> MLQFYRNLGKSGLRVSCL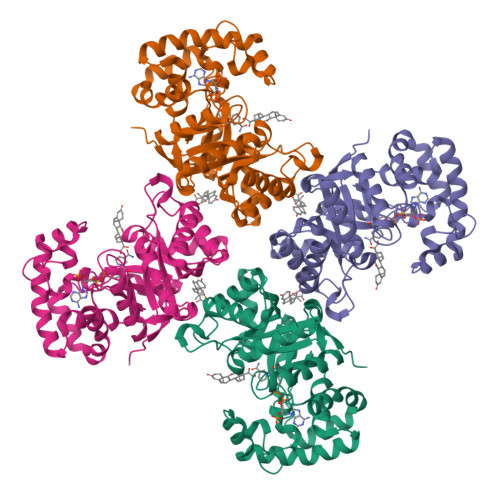GLGTWVTFGGQITDEMAEHLMTLAYDNGINLFDTAEVYAAGKAEVVLGNIIKKKGWRRSSLVITTKIFWGGKAETERGLSRKHIIEGLKASLERLQLEYVDVVFANRPDPNTPMEETVRAMTHVINQGMAMYWGTSRWSSMEIMEAYSVARQFNLIPPICEQAEYHMFQREKVEVQLPELFHKIGVGAMTWSPLACGIVSGKYDSGIPPYSRASLKGYQWLKDKILSEEGRRQQAKLKELQAIAERLGCTLPQLAIAWCLRNEGVSSVLLGASNAEQLMENIGAIQVLPKLSSSIVHEIDSILGNKPYS>GMSVPTTMFRLTGRDYPPAKLSHASLIIIDAQKEYLSGPLKLSGMDEAVANIARLLDAARKSGRPIIHVRHLGTVGGRFDPQGPAGQFIPGLEPLEGEIVIEKRMPNAFKNTKLHETLQELGHLDLIVCGFMSHSSVSTTVRRAKDYGYRCTLVEDASATRDLAFKDGVIPAAQIHQCEMAVMADNFACVAPTAS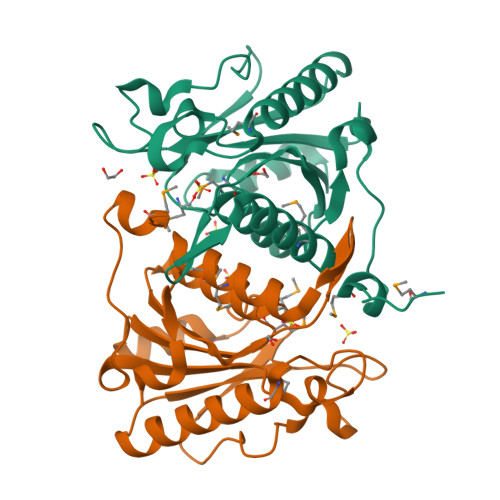LI[2x]2-[3-(morpholin-4-yl)propyl]-1H-benzo[de]isoquinoline-1,3(2H)-dione 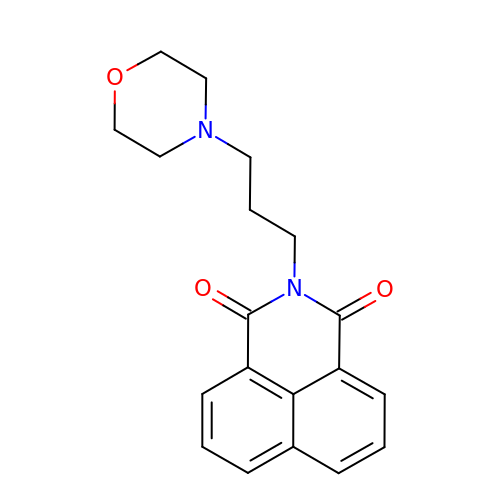| C19 H20 N2 O3 | GQPIEFFYGONFTJ-UHFFFAOYSA-N> MQEPLAAGAVILRRFAFNAAEQLIRDINDVASQSPFRQMVT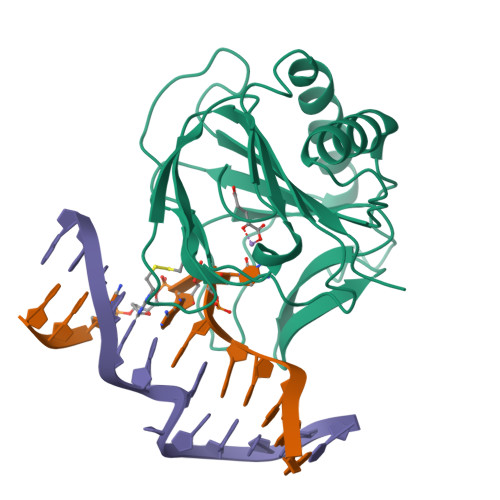PGGYTMSVAMTNCGHLGWTTHRQGYLYSPIDPQTNKPWPAMPQSFHNLCQRAATAAGYPDFQPDACLINRYAPGAKLCLHQDKDEPDLRAPIVSVSLGLPAIFQFGGLKRNDPLKRLLLEHGDVVVWGGESRLFYHGIQPLKAGFHPLTIDCRYNLTFRQAGKKE>[2x]MSLQRIVRVSLEHPTSAVCVAGVETLVDIYGSVPEGTEMFEVYGTPGVDIYISPNMERGRERADTRRWRFDATLEIIVVMNSPSNDLNDSHVQISYHSSHEPLPLAYAVLYLTCVDISLDCDLNCEGRQDRNFVDKRQWVWGPSGYGGILLVNCDRDDPSCDVQDNCDQHVHCLQDLEDMSVMVLRTQGPAALFDDHKLVLHTSSYDAKRAQVFHICGPEDVCEAYRHVLGQDKVSYEVPRLHGDEERFFVEGLSFPDAGFTGLISFHVTLLDDSNEDFSASPIFTDTVVFRVAPWIMTPSTLPPLEVYVCRVRNNTCFVDAVAELARKAGCKLTICPQAENRNDRWIQDEMELGYVQAPHKTLPVVFDSPRNGELQDFPYKRILGPDFGYVTREPRDRSVS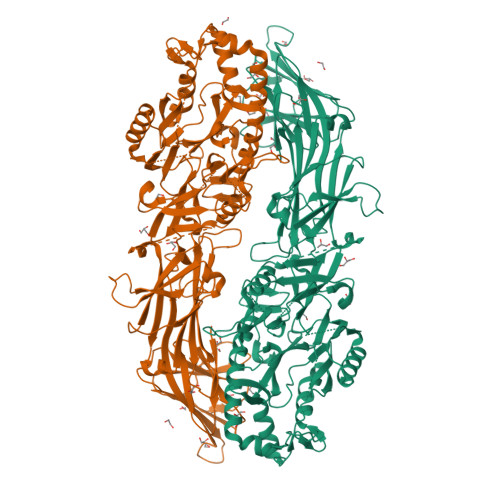GLDSFGNLEVSPPVVANGKEYPLGRILIGGNLPGSSGRRVTQVVRDFLHAQKVQPPVELFVDWLAVGHVDEFLSFVPAPDGKGFRMLLASPGACFKLFQEKQKCGHGRALLFQGVVDDEQVKTISINQVLSNKDLINYNKFVQSCIDWNREVLKRELGLAECDIIDIPQLFKTERKKATAFFPDLVNMLVLGKHLGIPKPFGPIINGCCCLEEKVRSLLEPLGLHCTFIDDFTPYHMLHGEVHAGTNVCRKPFSFKWWNMVP>[11x]AATTVNGGTVHFKGEVVNAACAVDAGSVDQTVQLGQVRTASLAQEGATSSAVGFNIQLNDCDTNVASKAAVAFLGTAIDAGHTNVLALQSSAAGSATNVGVQILDRTGAALTLDGATFSSETTLNNGTNTIPFQARYFATGAATPGAANADATFKVQYQ

Following this pattern, the type 1 pilus usher (FimD) and chaperone (FimC) help type 1 pili assemble into a composite pilus structure consisting of a short tip fibrillum made up of the adhesin protein (FimH) and two minor subunits (FimG and FimF) that is joined to the pilus rod, a homopolymer of ~1000 FimA subunits. Once extruded to the extracellular surface, the type 1 pilus coils into a rigid right-handed helical structure that is capable of unwinding into a flexible linear fiber. This ability to transition between a coiled, helical rod and a linear fiber has been proposed to allow the type 1 pilus to act as a ‘molecular spring’ to maintain adherence in the face of fluid shear forces. FimA is critical for proper assembly of the type 1 pilus and, as the major subunit that makes up the pilus rod, is also critical for the proper display of the FimH adhesin.

To characterize FimA polymers that form the type 1 pilus rod, we solved the cryo-EM structure of native type 1 pili appearing in a preparation of recombinantly expressed Type IV pili (T4P) from the E. coli K12 strain BW25113. The FimA reconstruction had an overall resolution of 4.2 Å, which is sufficient to build an atomic model of the structure. Overall, the type 1 pilus is a 70 Å diameter rod where each adjacent subunit rotates around the helical axis by 115° and translates along the axis by 7.7 Å. If we label each subunit along the 1-start helix by N, a subunit N0 interacts with six adjacent subunits (N-1,N-2,N-3,N+1,N+2,N+3). Further, in the structure we observe the N-terminal donor strand of one subunit completing the β-sheet of the adjacent subunit. Most prominently, the hydrophobic amino acids Val5, Val10 and Phe12 in the N-terminal β-strand (Nte) of one subunit are inserted into the next subunit’s hydrophobic groove created by a missing β-strand. Within the cryo-EM rod FimA structure, residues 25–29 adopt a helical conformation and residues 30–33 form a β-strand interaction with residues 10–13 from the Nte of the next FimA subunit. We can explain this by the fact that Ala22 in our rod model is tightly packed against Ala93 from another subunit and Val37 from a third subunit. Pili formed with the WT FimABW25113 protein require more than twice the force to unwind than the pili formed by the FimA BW25113 variant with an A22R mutation (~30 pN vs. 11pN), likely due to steric clashes caused by this substitution affecting the tightly packed interface between subunits. Interestingly, the non-conserved residues within the FimA sequences are all located on the exterior surface of the solved cryo-EM model, which is likely indicative of immune pressures selecting for antigenic diversification.>[2x]MMLSLNNLQNIIYNPVIPFVGTIPDQLDPGTLIVIRGH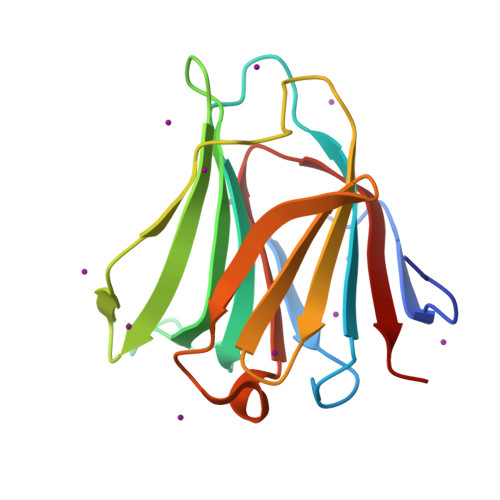VPSDADRFQVDLQNGSSVKPRADVAFHFNPRFKRAGCIVCNTLINEKWGREEITYDTPFKREKSFEIVIMVLKDKFQVAVNGKHTLLYGHRIGPEKIDTLGIYGKVNIHSIGFSFS>GPLGSPEFSKTKPFTLPILTIGELTNSRFPAPIDQLYTSPNADVVVQPQNGRCSLDGELQGTTQLLTTAICSYRGMTSNPTRDYWDGHLLHLVHPNGATYDPTEDVPAPFGTQDFRGILYGVLTQNPRASGDEAANSQGVYISSTSEKFTPKLGTIGLHQVQGNIASNQQSKFTPVGIAVNGNTPFRQWELPNYSGALTLNTNLAPAVGPNFPGEQILFFRSNVPSVQGGQPIEIDCLIPQEWVSHFYQESAPSQSDVALVRYVNPDTGRTIFEA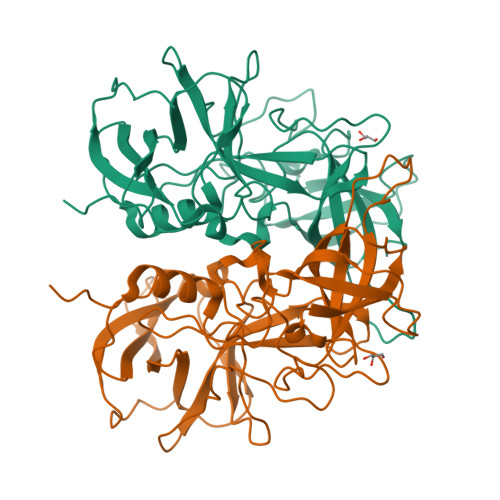KLHRQGFITIAATGSNPVVVPPNGYFRFDSWVNQFYALAPM[2x]>ASQNSFRIEYDTFGELKVPNDKYYGAQTVRSTMNFKIGGVTERMPTPVIKAFGILKRAAAEVNQDYGLDPKIANAIMKAADEVAEGKLNDHFPLVVWQTGSGTQTNMNVNEVISNRAIEMLGGELGSKIPVHPNDRVNKSQSSNDTFPTAMHIAAAIEVHEVLLPGLQKLHDALDAKSKEFAQIIKIGRTHTQDAVPLTLGQEFSGYVQQVKYAMTRIKAAMPRIYELAAGGTAVGTGLNTRIGFAEKVAAKVAALTGLPFVTAPNKFEALAAHDALVELSGAMNTTACSLMKIANDIRFLGSGPRSGLGELILPENEPGSSIMPGKVNPTQCEAMTMVAAQVMGNHVAVTVGGSNGHFELNVFKPMMIKNVLHSARLLGDASVSFTENCVVGIQANTERINKLMNESLMLVTALNPHIGYDKAAKIAKTAHKNGSTLKETAIELGYLTAEQFDE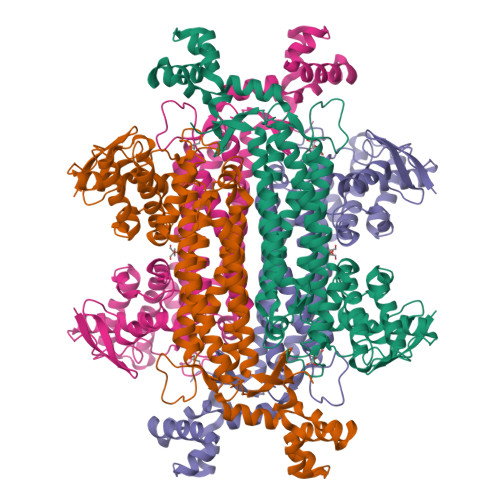WVKPKDMLGPK[2x]N-[(naphthalen-1-ylamino)(oxo)acetyl]-beta-D-glucopyranosylamine | C18 H20 N2 O7 | 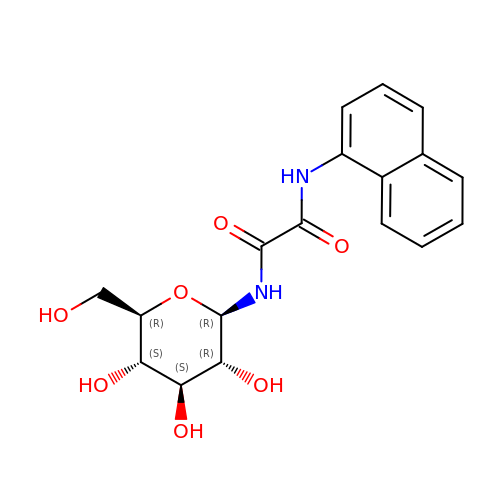AHNFLCXLAFQOCX-VPKNTQAGSA-N> MNCRSEVLEVSVEG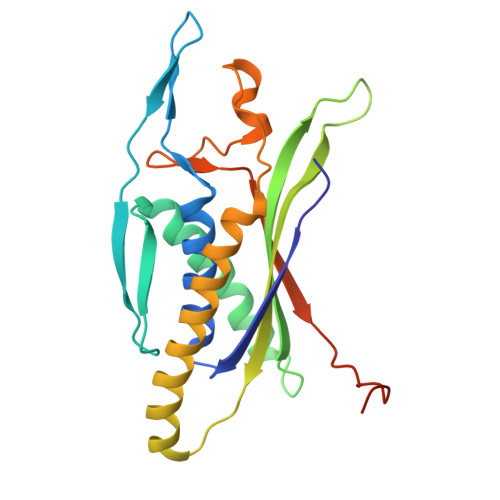RQVEEAMLAVLHTVLLHRSTGKFHYAAAGTYSIGTVGTQDVDCDFIDFTYVRVSSEELDRALRKVVGEFKDALRNSGGDGLGQMSLEFYQKKKSRWPFSDECIPWEVWTVKVHVVALATEQERQICREKVGEKLCEKIINIVEVMNRHEYLPKMPTQSEVDNVFDTGLRDVQPYLYKISFQITDALGTSVTTTMRRLIKDTLAL> MVPISPIETVPVKLKPGMDGPKVKQWPLTE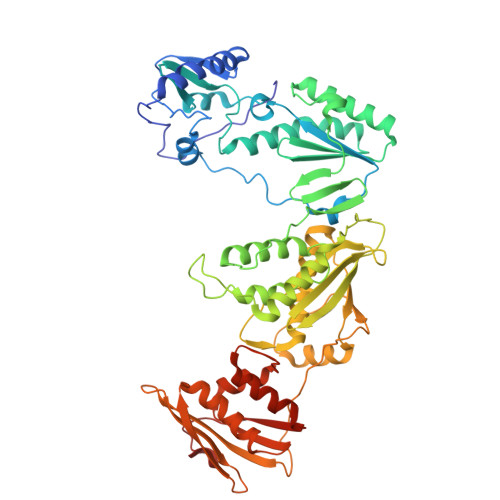EKIKALVEICTEMEKEGKISKIGPENPYNTPVFACKKKDSTKWRKLVDFRELNKRTQDFWEVQLGIPHPAGLKKKKSVTVLDVGDAYFSVPLDEDFRKYTAFTIPSINNETPGIRYQYNVLPQGWKGSPAIFQSSMTKILEPFKKQNPDIVIYQYMDDLYVGSDLEIGQHRTKIEELRQHLLRWGLTTPDKKHQKEPPFLWMGYELHPDKWTVQPIVLPEKDSWTVNDIQKLVGKLNWASQIYPGIKVRQLSKLLRGTKALTEVIPLTEEAELELAENREILKEPVHGVYYDPSKDLIAEIQKQGQGQWTYQIYQEPFKNLKTGKYARMRGAHTNDVKQLTEAVQKITTESIVIWGKTPKFKLPIQKETWETWWTEYWQATWIPEWEFVNTPPLVKLWYQLEKEPIVGAETFYVDGAANRETKLGKAGYVTNKGRQKVVPLTNTTNQKTELQAIYLALQDSGLEVNIVTNSQYALGIIQAQPDKSESELVNQIIEQLIKKEKVYLAWVPAHKGIGGNEQVDKLVSA> MNTVDVNMMDNNPAARLEELRTIMKKNKIDVYILINSDEHNSEIINEKDKKIVKITNYSGADGILIVTKDKPILYVNALYELQAMNELDQNLFTLRISRIDNRDEIFETISSLEFNTIAFDGKNTSVVFYEKLRKALLNAYPKKKIVEKIIYNNNFDDVNKKDDENVLNFLVLEKSLVEIKDYPVNNKTLYIHDRKYNGACAGEKIDKLKQSLMYDIKNVDNLLLSELDEIAYLLNLRGYDYQYSPLFYSYLLFQFDREEQDFSKIVFFTTVKNLPADVKNLLEINKVIVKEYEEIVPYLRDVVIPSIPKHNDDNPDFKKYDISLSPYINLMIYKLFDRKNVLLQNSPVVKMKAVKNDVEIDNMKQAHILDGLALLQFFHWCEQKRKTKELFNETEMSLRHKVDYFRSTKKNFIFPSFSTISASGPNAAVIHYECTDKTNATIKPAIYLLDSGGQYLHGTTDVTRTTHFGEPTAEEKRIYTLVLKGHLRLRKVIFASYTNSSALDFIARENLFNNFMDYNHGTGHGVGLTLNVHEGGCSIGPVGGAPLKKNMVLSNEPGYYMKDKFGVRIENMQYVISKEITDTTEYLSFDDLTMYPYEKKLLDFSLLTNQEIKELNEYHTTI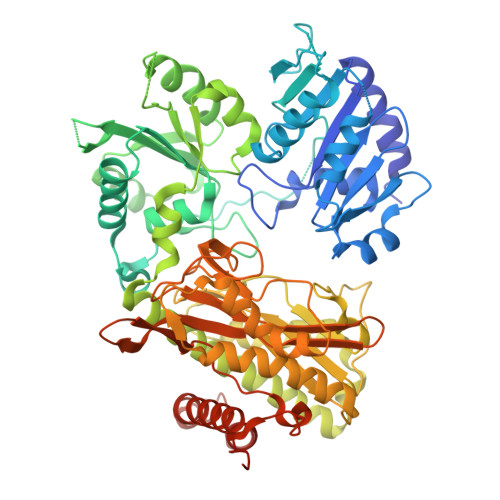RNTLLPLVKQSPQEYGESVEKYLIEITEPIAIHNNHHHHHH> QTSVSPSKVILPRGGSVLVTCSTSCDQPMLLGIETPLPKKELLLPGNNRKVYELSNVQEDSQPMCYSNCPDGQSTAKTFLTVYWTPERVELAPLPSWQPVGKNLTLRCQVEGGAPRANLTVVLLRGEKELKREPAVGEPAEVTTTVLVRRDHHGANFSCRTELDLRPQGLELFENTSAPYQLQTFVLPATPPQLVSPRVLEVDTQGTVVCSLDGLFPVSEAQVHLALGDQRLNPTVTYGNDSFSAKASVSVTAEDEGTQRLTCAVILGNQSQETLQTVTIYSFPAPNVILTKPEVSEGTEVTVKCEAHPRAKVTLNGVPAQPLGPRAQLLLKATPEDNGRSFSCSATLEVAGQLIHKNQTRELRVLYGPRLDERDCPGNWTWPENSQQTPMCQAWGNPLPELKCLKDGTFPLPIGESVTVTRDLEGTYLCRARSTQGEVTRE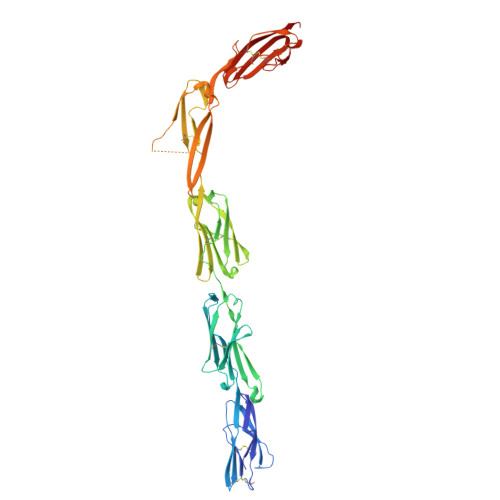VTVNVLSP> HMGTGSLGGGFPGKGMKIVTSFYPIYAMVKEVSGDLNDVRMIQSSSGIHSFEPSANDIAAIYDADVFVYHSHTLESWAGSLDPNLKKSKVKVLEASEGMTLERVPGLEDVEAGDGVDEKTLYDPHTWLDPEKAGEEAQIIADKLSEVDSEHKETYQKNAQAFIKKAQELTKKFQPKFEKATQKTFVTQHTAFSYLAKRFGLNQLGIAGISPEQEPSPRQLTEIQEFVKTYKVKTIFTESNASSKVAETLVKSTGVGLKTLNPLQSDPQNDKTYLENLEENMSILAEELKG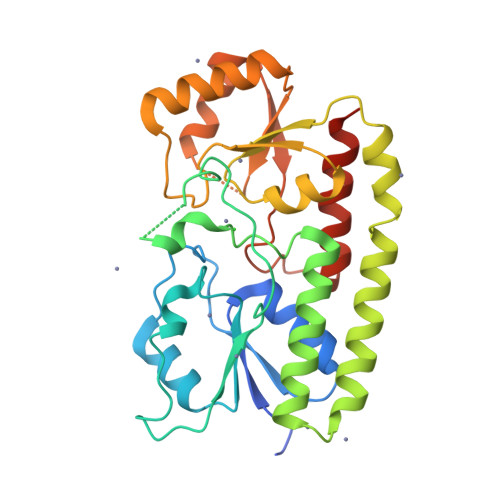NLYFQ>GSMFTDWHEAAIGKTHNRMNFDCGDADLNQFLQRHARQNHEKGTTKTYVALDNSDVTRIHGFYSVSPASLIYAQVPGAISKGLGRYDVPVFRLGRLAVDKSMQGQGLGAQLLLSAGKRCIQAALQVGGVALLIDAKNKQVCD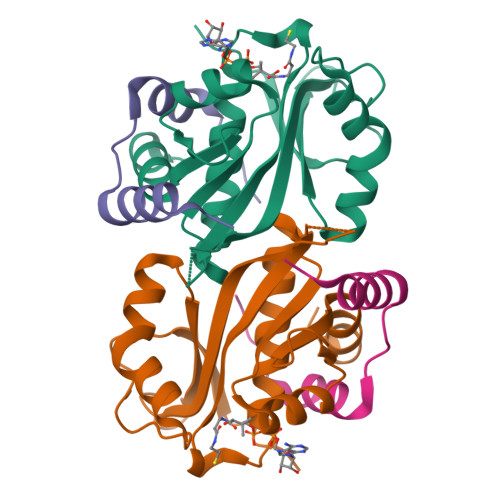WFKGFGAVPLNDQPLSLLLSFKTLYAALSASGRL[2x];>[2x]YLTERDTKMIMEILDNPPAPNEKLLAAAFALPDMKK> MHHHHHHVMIMKAFISENVRGIYAFDENGNLIEKRYFTDKPEKVLDQLLKGEITKDLEELLNSLKEKGYDEFVFEHPELSRRAKELGFSATTEFPNIAGERLRSNPEEFLGENWFEEYYKVGVALTRMRIQEQS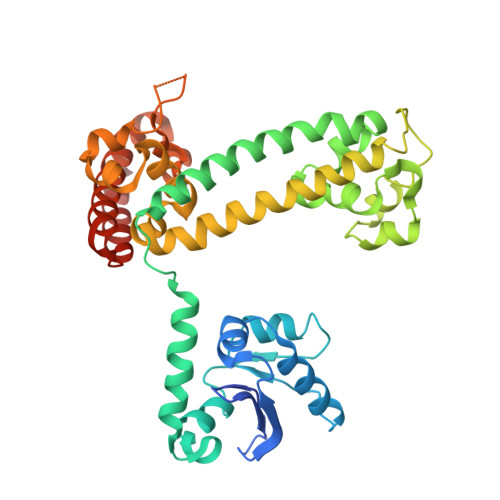GARDKMVIQAIEALDDINLLVARLREWYSLHFPELDELLPKHPQYVAFVKTVGHRDNINEEVLRELGLSEEKIKKILEAKEKTMGAWMDQTDIEVVRQLAEEIQLRKKLEDYIDRAMDDVAPNLKALVGAKLAARLISLAGGLRELAMMPSSTIQVLGAEKALFRHLRTGAKPPKHGVIYQYPAINRSPWWQRGKIARALAGKLAIAARVDYFSGEYIAEELKKELEARIREIKEKY>[4x]MTLLTNAEEISDIAFGFMGSKALFAALHHGVFTCLADGPLSVEEMAAATGL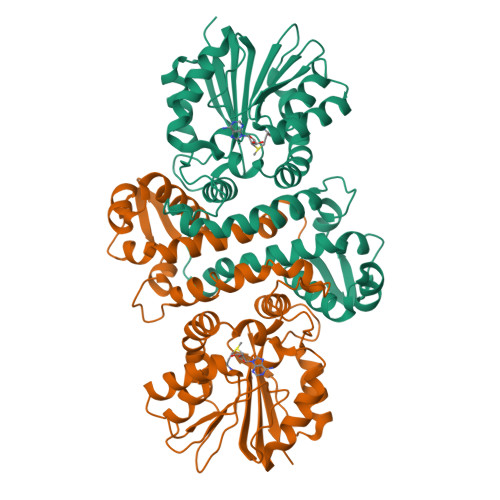HPDRVQTLLTALASLGVVSAVEGRFANSPAAESFLVKGAKYDFGDYLRLQVDRQMYGLLDQIEDAIANNLPDDATSSYADWFSDPEQAKLYSNSQHAGSLGPARGLAKLIDLSGGKKLLDVGGGTGAFAITLCKAFADLAATIVDFPNVAALGKGYVEKAGLSDRIEYVIGDALRTEWPREQDAILMSYLFSGVAGDEHDSLLKRAYDHLVPGGRLLIHDFVVTADRTGPKLAALWQLQHTAFTPEARSLDDEWLAEQLKKTGFTDVKVGPMIPGMTMLAEAVRPE N-ACRIDIN-9-YL-N'-[3-(ACRIDIN-9-YLAMINO)PROPYL]PROPANE-1,3-DIAMINE | C32 H31 N5 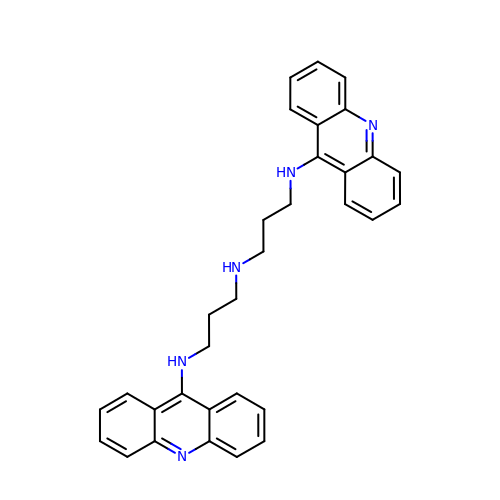| WGBHBVVVCBOHMA-UHFFFAOYSA-N>MEEELVVISKSIVNPRSLKKPTSVKKIQLTPWDLSRLRFGYLQRGLLFHKIEVKQLQASLSVALDRFYPLAGRLVKLKNDDDTVSFFISCDGSGVEFVHAVAKNIELSDVLELSGSVPGFFASFFPATGIKNYHGVSRSLLMVQVTEMKDGVFIGFGYNSTVADATSIWKFINAWSEICSKDSSGSQTFQRRLHLKGWFFDEIDYPIHIPDPETKPTSYVTTPTNLQEKMFHVTKENVLKLDAKANDEADQKISSIQAVLAYIWRSMVKHSGMSREEETHCRLPINMRQRLNPPLEEE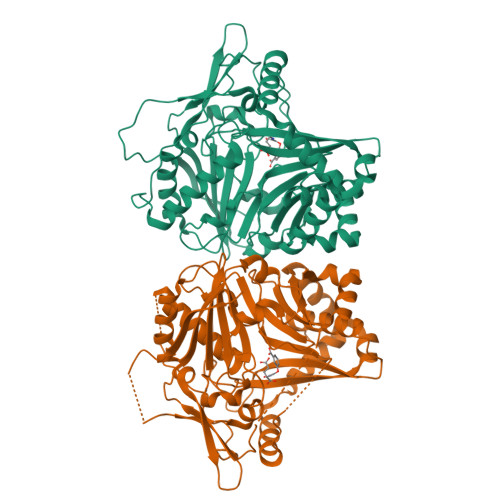CFGNVSQTGIATVTVGELLDHGLGWAAMQINNMELSQTDEKAKAFAENWVKNIKIPVSVGSKDLVVTNSHRFDVYCNDFGWGKPIAARAGPPYLNGRLVVFKGIGEASLDFQACLLPQVVEKLVKDAEFNEYVSIV[2x]PERIODATE | I O4 | 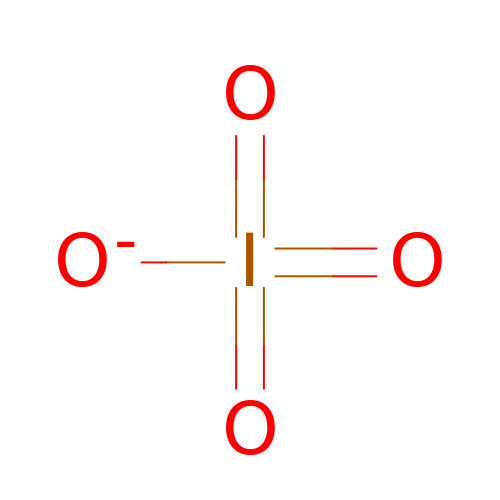KHIWWQKSHDUIBK-UHFFFAOYSA-M> TLTEDLDAPQDTGNIENGAADNSPQPRTTFDYTGNPLPPDTKLENFFSFYRLLPMGGSGAPSLSFPADEGTIIPLNPINWLKGADVSGIAAML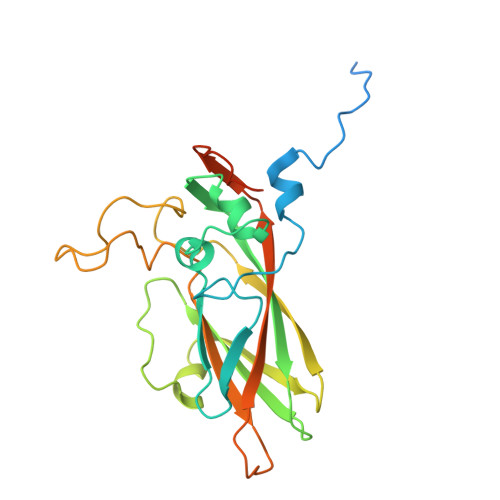SCFTYIAADLRITLRFSNPNDNPATMLVAFAPPGATIPLKPTRQMLSNFYMAEVPVSAATSTMVSFSIPYTSPLSAIPTSYFGWEDWSGTNFGQLSSGSWGNLMLIPSLSVDSAIPFDFQLSCWVAFGNFKAWVPRPPPPLPPLPTPAANAERTVAVIKQ>MTLVKIGLWGGNGGSAQDISVPPKKLLGVTIYSSDAIRSIAFNYIGVDGQEYAIGPWGGGEGTSTEIKLGSSEHIKEISGTHGPVYDLADIVTYL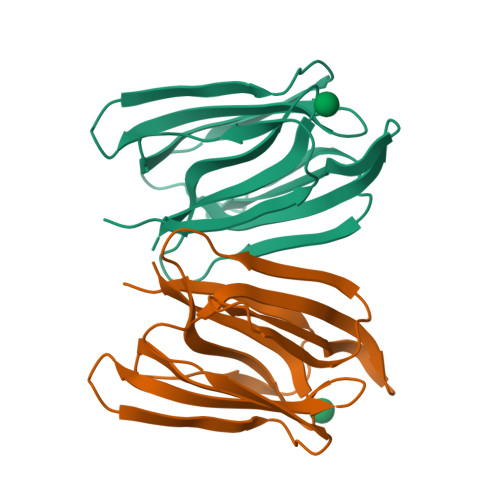KIVTSANNTYEAGVPNGKEFSIPLQDSGHVVGFFGRSGTLIDAIGIYVHP[2x]> MLSRKGIIPEEYVLTRLAEDPTEPRYRTRERRARFVSKKGNCNVAHKNIREQGRFLQDVFTTLVDLKWPHTLLIFTMSFLCSWLLFAMVWWLIAFAHGDLAPGEGTNVPCVTSIHSFSSAFLFSIEVQVTIGFGGRMVTEECPLAILILIVQNIVGLMINAIMLGCIFMKTAQAHRRAETLIFSKHAVITLRHGRLCFMLRVGDLRKSMIISATIHMQVVRKTTSPEGEVVPLHQVDIPMENGVGGNSIFLVAP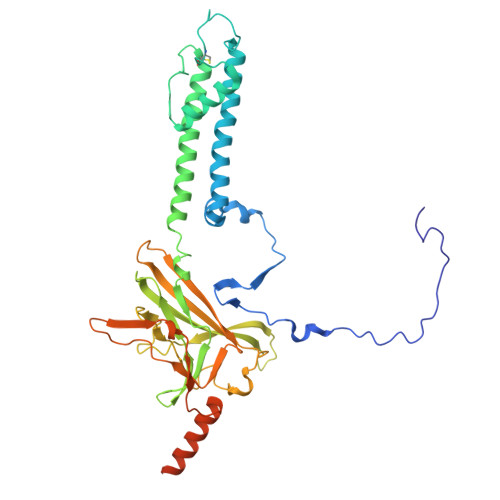LIIYHVIDSNSPLYDLAPSDLHHHQDLEIIVILEGVVETTGITTQARTSYLADEILWGQRFVPIVAEEDGRYSVDYSKFGNTVKVPTPLCTARQLDEDRSLLDALTLASSRGPLRKRSVAVAKAKPKFSISPDSLS>MAKKTSSKGKLPPLAPGFLHLLQPDLPIYLLGLTQKFGPIYRLHLGLQDVVVLNSKRTIEEAMVKKWADFAGRPEPLTYKLVSRNYPDLSLGDYSLLWKAHKKLTRSALLLGIRDSMEPVVEQLTQEFCERMRAQPGTPVAIEEEFSLLTCSIICYLTFGDKIKDDNLMPAYYKCIQEVLKTWSHWSIQIVDVIPFLRFFPNPGLRRLKQAIEKRDHIVEMQLRQHKESLVAGQWRDMMDYMLQGVAQPSMEEGSGQLLEGHVHMAAVDLLIGGTETTANTLSWAVVFLLHHPEIQQRLQEELDHELGPGASSSRVPYKDRARLPLLNATIAEVLRLRPVVPLALPHRTTRPSSISGYDIPEGTVIIPNLQGAHLDETVWERPHEFWPDRFLEPGKNSRALAFGCGARVCLGEPLARLELFVVLTRLLQAFTLLP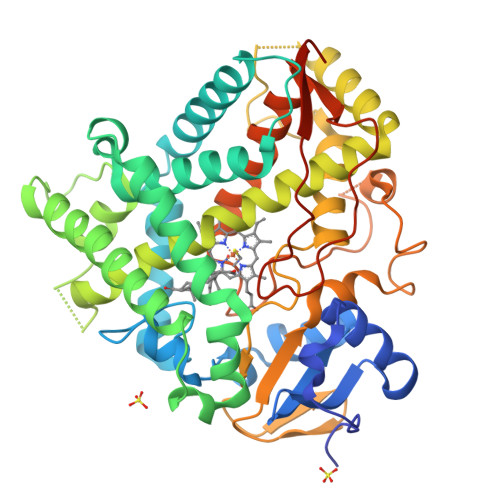SGDALPSLQPLPHCSVILKMQPFQVRLQPRGMGAHSPGQSQHHHHHH[3x]>[4x]SNAMSDKFHIL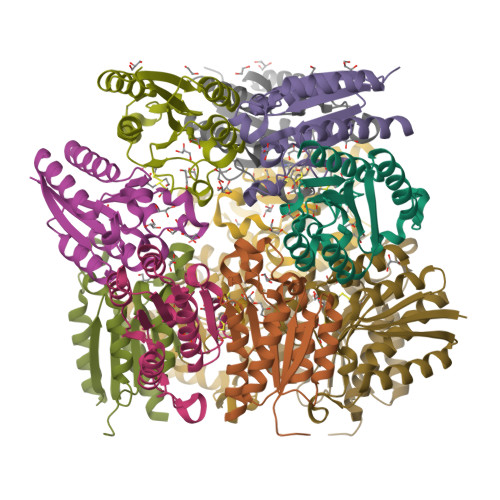LLNGPNLNLLGTREPEKYGYTTLAEIVSQLEIQAQGMDVALSHLQSNAEHALIDSIHQARGNTDFILINPAAFTHTSVALRDALLGVQIPFIEIHLSNVHAREPFRHHSYLSDIAVGVICGLGADGYNFALQAAVNRLSKSN> MVVLDKKLLERLTSRKVPLEELEDMEKRCFLSTFTYQDAFDLGTYIRNAVKENFPEKPVAIDISLPNGHCLFRTVTYGGSALDN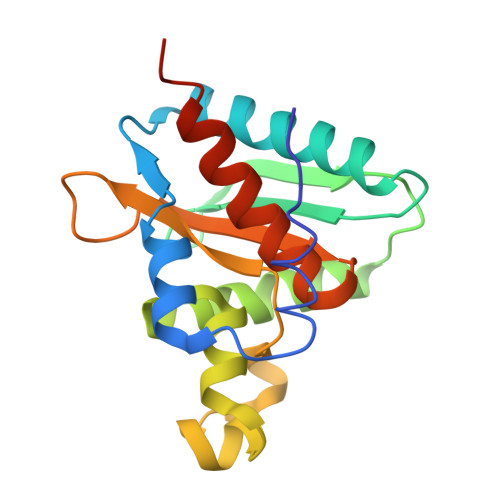DFWIQRKKKTALRFGHSSFYMGCKKGDKTPEEKFFVDSKEYAFHGGAVLIQSERSDYPYACLTISGLKQEEDHLMAVSSLIAFANESLEEDLNLD4-(ACETYLAMINO)-5-AMINO-3-HYDROXYBENZOIC ACID | C9 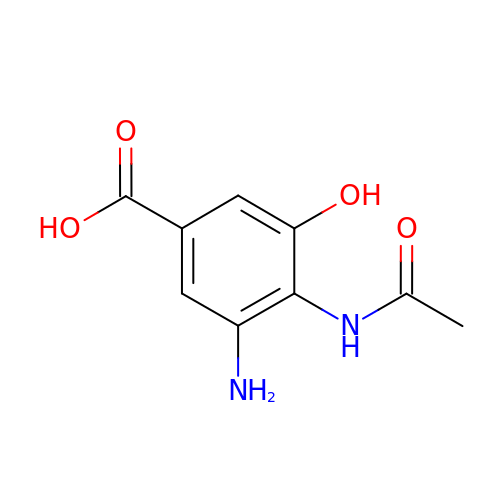H10 N2 O4 | CALDTVBHJMBRTM-UHFFFAOYSA-N Glycoprotein 130 (gp130) is a signaling receptor shared by interleukin-6 (IL-6) family cytokines (or gp130 family cytokines), including IL-6, ciliary neurotrophic factor (CNTF), cardiotrophin-like cytokine factor 1 (CLCF1), leukemia inhibitory factor (LIF), oncostatin M (OSM), cardiotrophin-1 (CT-1), IL-11, IL-27, IL-35, and IL-39 (1). These cytokines share a canonical four-helix bundle structure in which four major helices (termed helices A to D) are linked by three loops (termed AB, BC, and CD loops), as well as three conserved receptor binding epitopes (termed sites 1 to 3). IL-6 and IL-11 signal through gp130 homodimerization, while other cytokines require another “tall” signaling receptor, such as LIF receptor (LIFR) or IL-27 receptor subunit alpha (IL-27Rα), which forms a heterodimer with gp130 for signal transduction. The extracellular domains (ECDs) of gp130 include an N-terminal immunoglobulin (Ig)–like domain (D1), a cytokine-binding homology region (CHR, D2D3), and three membrane-proximal fibronectin type III domains (FNIII, D4 to D6).

In addition, we have solved a 3.40-Å cryo-EM structure of the CRLF1-CLCF1-CNTFRα complex, which exhibits an unexpected 2:2:2 stoichiometry. The two CNTFRα molecules bind to site 1 of the two CLCF1 ligands without contacting CRLF1, indicating that CNTFRα may not be essential for CLCF1-mediated CRLF1 dimerization. The elbow region of CRLF1 D2D3 engages CLCF1 site 2 mimicking the interactions between gp130 D2D3 and CLCF1. Therefore, the CRLF1-CLCF1 interface has a much larger buried surface area (1480 Å2) than the gp130-CLCF1 interface (944 Å2). Notably, the three gp130 residues crucial for engaging CLCF1, W164, F191, and D215 all have equivalents in CRLF1 at similar locations, i.e., W177, F204, and D228, respectively. Furthermore, the way LIFR D3 captures CLCF1 site 3 is copied by D1 of another CRLF1 molecule, CRLF1′, in the CRLF1-CLCF1-CNTFRα complex. CLCF1 F178 is stacked against CRLF1′ G126′ and is surrounded by N113′, V115′, I123′, and C128′ of CRLF1′, while CLCF1 K181 coordinates with S110′, N113′, and C128′ of CRLF1′ to form hydrogen bonds. The two CRLF1 molecules also directly contact each other at their D3 domains. While R245 of one CRLF1 couples to E279 of another CRLF1 to form hydrogen bonds and salt bridges, H332, A335, and V306 from one molecule pack against the same corresponding residues from another molecule to hold both CRLF1 D3 domains together. Unexpectedly, CLCF1 sites 2 and 3 are engaged by two CRLF1 molecules analogous to how they are engaged by gp130 and LIFR in the CLCF1 signaling complex, supporting the model that CLCF1 has to dissociate from CRLF1 to bind to gp130 and LIFR to form a functional signaling complex.

>[2x]AHTAVISPQDPTLLIGSSLLATCSVHGDPPGATAEGLYWTLNGRRLPPELSRVLNASTLALALANLNGSRQRSGDNLVCHARDGSILAGSCLYVGLPPEKPVNISCWSKNMKDLTCRWTPGAHGETFLHTNYSLKYKLRWYGQDNTCEEYHTVGPHSCHIPKDLALFTPYEIWVEATNRLGSARSDVLTLDILDVVTTDPPPDVHVSRVGGLEDQLSVRWVSPPALKDFLFQAKYQIRYRVEDSVDWKVVDDVSNQTSCRLAGLKPGTVYFVQVRCNPFGIYGSKKAGIWSEWSHPTAASTPRSERPGPGGGACEPRGGEPSSGPVRRELKQFLGWLKKHAYCSNLSFRLYDQWRAWMQKSHKTRNQDEGILPSGRRGTARGPARHHHHHHHHHH;>QRHSPQEAPHVQYERLGSDVTLPCGTANWDAAVTWRVNGTDLAPDLLNGSQLVLHGLELGHSGLYACFHRDSWHLRHQVLLHVGLPPREPVLSCRSNTYPKGFYCSWHLPTPTYIPNTFNVTVLHGSKIMVCEKDPALKNRCHIRYMHLFSTIKYKVSISVSNALGHNATAITFDEFTIVKPDPPENVVARPVPSNPRRLEVTWQTPSTWPDPESFPLKFFLRYRPLILDQWQHVELSDGTAHTITDAYAGKEYIIQVAAKDNEIGTWSDWSVAAHATPWTEEPRHLTTEAQAAETTTSTTSSLAPPPTTKICDPGELGSEQKLISEEDLGGEQKLISEEDLHHHHHH[2x];>LNRTGDPGPGPSIQKTYDLTRYLEHQLRSLAGTYLNYLGPPFNEPDFNPPRLGAETLPRATVDLEVWRSLNDKLRLTQNYEAYSHLLCYLRGLNRQAATAELRRSLAHFCTSLQGLLGSIAGVMAALGYPLPQPLPGTEPTWTPGPAHSDFLQKMDDFWLLKELQTWLWRSAKDFNRLKKKMQPPAAAVTLHLGAHGFHHHHHH[2x]Here we describe the determination of the crystal structure of CinA from T. thermophilus (TtCinA), which contains both the NMN deamidase and COG1058 domains and is therefore a bifunctional enzyme. In addition, we show that TtCinA adopts a three-domain structure, with a third, previously unidentified, KH-type domain between the NMN deamidase and COG1058 domains. We demonstrate that TtCinA adopts an asymmetric dimer and present structures with NCN, ADP-ribose, AMP, and ATP bound, which provide experimental validation for the modes of substrate binding proposed previously. We use these structures to propose models for both enzymatic activities and suggest that large scale movement of the COG1058 domains is linked to ADPR catalysis as well as providing a rationale for the usual asymmetric arrangement of the TtCinA dimer.

The complete structure forms a dimer, with an overall oval shape. It was readily apparent that each chain comprises three, not two, domains; the third domain sits between the NMN deamidase (NMD) and COG1058 domains. It forms a KH-type fold, with two α-helices packed against a three-stranded β-sheet (referred to hereafter as the “KH domain”). Most strikingly, the TtCinA dimer is asymmetric; the NMD and KH domains are related by a common 2-fold symmetry axis, which runs horizontally along the main axis of the complex. These two domains superpose between the two chains with a root mean square deviation of 1.1 Å. The KH and NMD domains of chain A form a buried surface area of 815 Å2 with the COG1058 domain of chain B, whereas the value for the inverse, i.e. the KH/NMD of chain B contacting COG1058 of chain A, is 57 Å2 (calculations were performed using PISA). Critically, the asymmetry in contacts made by the COG1058 domain results in a difference in the environments of the ADPR active sites on each chain (discussed further below). The formation of a TtCinA dimer in the crystal was corroborated by measurement of molecular mass by size exclusion chromatography, which gave a value of ∼72 kDa, close to the predicted value of 86 kDa expected for a dimer (not shown).

>MERAEILGVGTELLYGETLDTNTAEIARSLKPYALKVERTLRVADEVAPLAREVEEAFARARLVVLSGGLGPTPDDVTREAVALALGEPLELDEAVLGEIEAFFRARGRAMPEANRKQAMRIPSATWLKNPRGTAPGWWVRKGGKDLVLLPGPPPEWRPMWQEVLPRLGLPRRPYAERVLKTWGIGESEIVERLGPLFVREEEVEVGTYPKVHGVEVVVRGREDRVAELAERIKKKLLKEVWGEGEMTLAEAVKRRMEREGATLSTMESLTGGLLGAEITRVPGASRFYLGGVVSYSVGAKARFGVPQDLLSRTVSAETARAMAEAARSLFGSTYALATTGVAGPDPLEGEPPGTVYVALAGPTGAEVRRYRFPGDRETVRLRSVYAALALLVT[2x]>MSNEDLKLKVAKEAVKLVKDGMVIGLGTGSTAALFIRELGNRIREEELTVFGIPTSFEAKMLAMQYEIPLVTLDEYDVDIAFDGADEVEETTLFLIKGGGGCHTQEKIVDYNANEFVVLVDESKLVKKLGEKFPIPVEVIPSAYRVVIRALSEMGGEAVIRLGDRKRGPVITDNGNMIIDVFMNIDDAIELEKEINNIPGVVENGIFTKVDKVLVGTKKGVKTLKK[4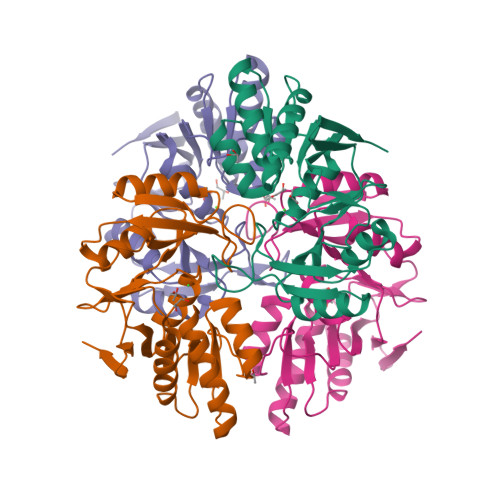x]>[6x]SYYHHHHHHLESTSLYKKAGLQRTLVLIKPDAFERSLVAEIMGRIEKKNFKIVSMKFWSKAPRNLIEQHYKEHSEQSYFNDNC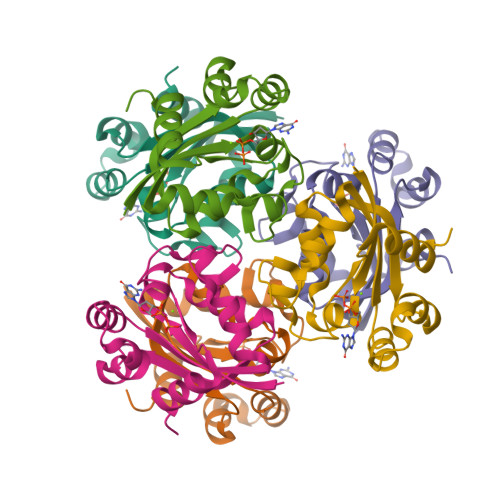DFMVSGPIISIVYEGTDAISKIRRLQGNILTPGTIRGDLANDIRENLIHASDSEDSAVDEISIWFPETKMETDN> XMEAFLGTWKMEKSEGFDKIMERLGVDFVTRKMGNLVKPNLIVTDLGGGKYKMRSESTFKTTECSFKLGEKFKEVTPDSREVASLITVENGVMKHEQDDKTKVTYIERVVEGNELKATVKVDEVVCVRTY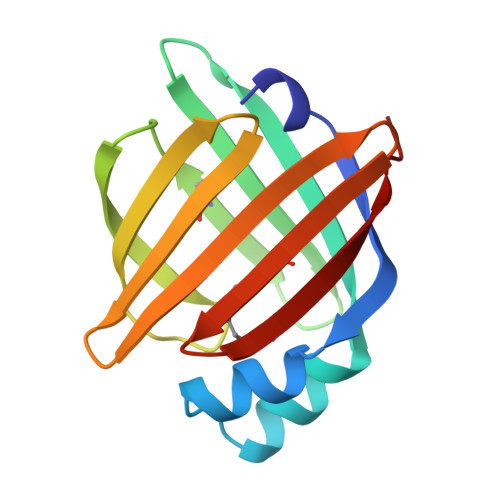SKVA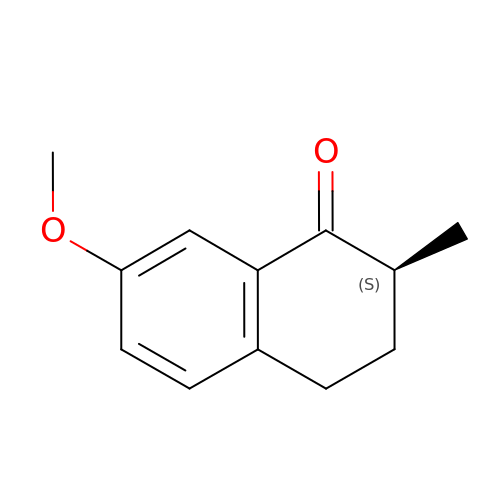(2S)-7-methoxy-2-methyl-3,4-dihydronaphthalen-1(2H)-one | C12 H14 O2 | YVPRDJIRFPVNJW-QMMMGPOBSA-N>[2x]GSHMTPTPRPTDGVDIYFGMPGEISEHEGFLRAKMDLEERRMRQINEVMREWAMADNQSKNLPKADRQ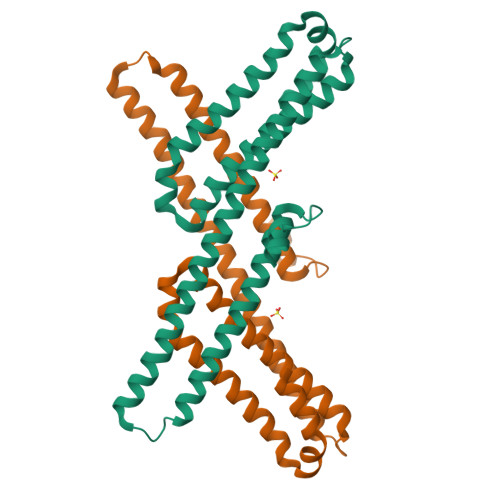ALNEHFQSILQTLEEQVSGERQRLVETHATRVIALINDQRRAALEGFLAALQADPPQAERVLLALRRYLRAEQKEQRHTLRHYQHVAAVDPEKAQQMRFQVHTHLQVIEERVNQSLGLLDQNPHLAQELRPQIQELLHSEHLGPSE> MTPLVKDIIMSSTRMPALFLGHGSPMNVLEDNLYTRSWQKLGMTLPRPQAIVVVSAHWFTRGTGVTAMETPPTIHDFGGFPQALYDTHYPAPGSPALAQRLVELLAPIPVTLDKEAWGFDHGSWGVLIKMYPDADIPMVQLSIDSSKPAAWHFEMGRKLAALRDEGIMLVASGNVVHNLRTVKWHGDSSPYPWATSFNEYVKANLTWQGPVEQHPLVNYLDHEGGTLSNPTPEHYLPLLYVLG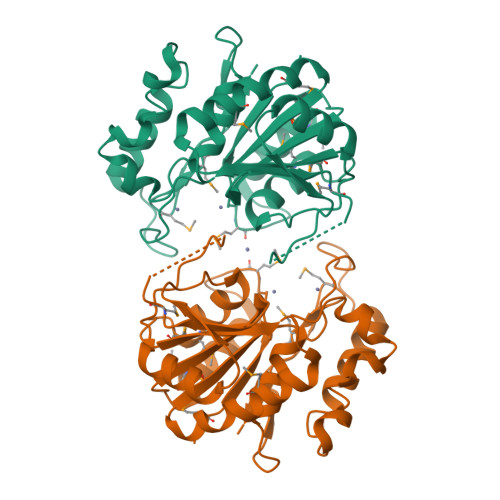AWDGQEPITIPVEGIEMGSLSMLSVQIG>[2x]GSHMDKLPIEETLEDSPQTRSLLGVFEEDATAISNYMNQLYQAMHRIYDAQNELSAATHLTSKLLKEYEKQRFPLGGDDEVMSSTLQQFSKVIDELSSCHAVLSTQLADAMMFPITQFKERDLKEILTLK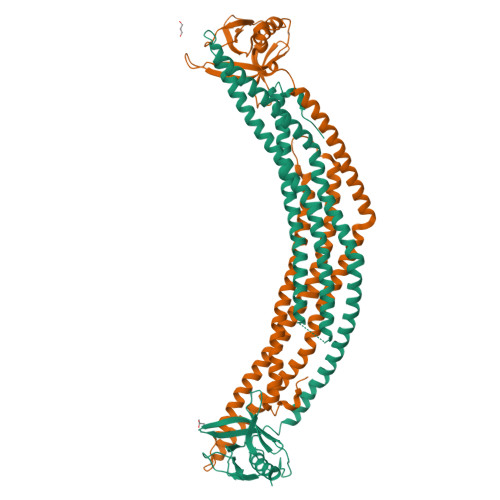EVFQIASNDHDAAINRYSRLSKKRENDKVKYEVTEDVYTSRKKQHQTMMHYFCALNTLQYKKKIALLEPLLGYMQAQISFFKMGSENLNEQLEEFLANIGTSVQNVRREMDSDIETMQQTIEDLEVASDPLYVPDPDPTKFPVNRNLTRKAGYLNARNKTGLVSSTWDRQFYFTQGGNLMSQARGDVAGGLAMDIDNCSVMAVDCEDRRYCFQITSFDGKKSSILQAESKKDHEEWICTINNISK;>[2x]MPAVDKLLLEEALQDSPQTRSLLSVFEEDAGTLTDYTNQLLQAMQRVYGAQNEMCLATQQLSKQLLAYEKQNFALGKGDEEVISTLHYFSKVVDELNLLHTELAKQLADTMVLPIIQFREKDLTEVSTLKDLFGLASNEHDLSMAKYSRLPKKKENEKVKTEVGKEVAAARRKQHLSSLQYYCALNALQYRKQMAMMEPMIGFAHGQINFFKKGAEMFSKRMDSFLSSVADMVQSIQVELEAEAEKMRVSQQELLSVDESVYTPDSDVAAPQINRNLIQKAGYLNLRNKTGLVTTTWERLYFFTQGGNLMCQPRGAVAGGLIQDLDNCSVMAVDCEDRRYCFQITTPNGKSGIILQAESRKENEEWICAINNISR>GAMATQAPTFTQPLQSVVVLEGSTATFEAHISGFPVPEVSWFRDGQVKLERLPGVQISFSDGRAKLTIPAVTKANSGRYSLKATNGSGQATSTAELLVKAETAPPNFVQRLQSMTVRQGSQVRLQVRVTGIPTPVVKFYRDGAEIQSSLDFQISQEGD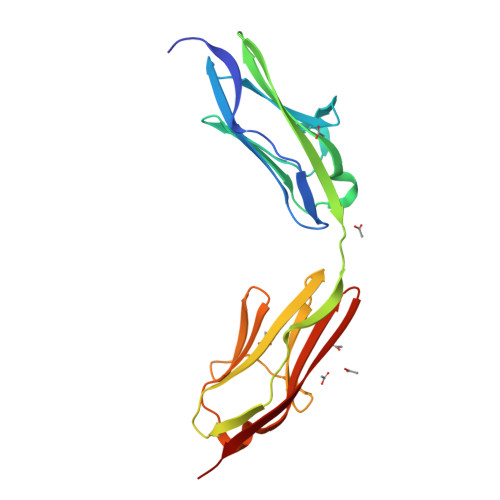LYSLLIAEAYPEDSGTYSVNATNSVGRATSTAELLVQGE[5x]> GPGSSSEST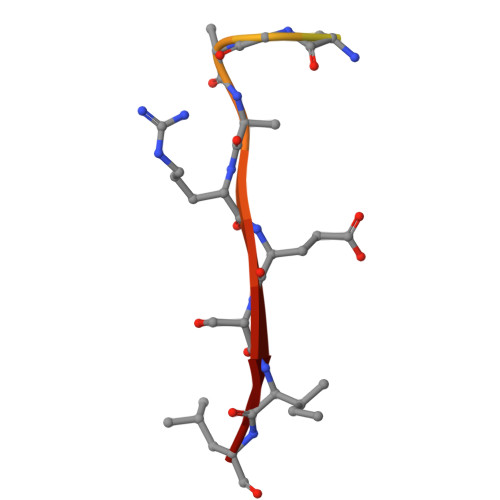GFGEERESIL>[2x]MAAKPKLYYFNGRGRMESIRWLLAAAGVEFEEEFLETREQYEKMQKDGHLLFG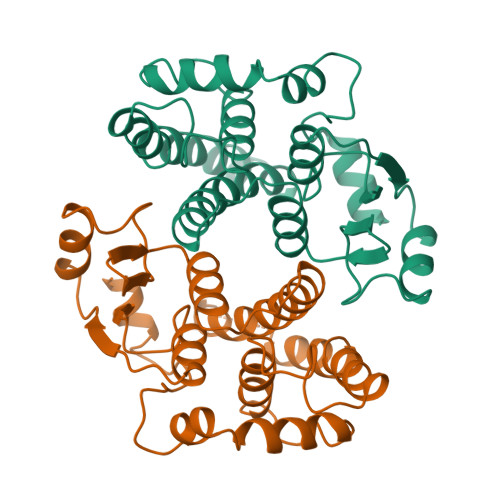QVPLVEIDGMMLTQTRAILSYLAAKYNLYGKDLKERVRIDMYADGTQDLMMMIAVAPFKTPKEKEESYDLILSRAKTRYFPVFEKILKDHGEAFLVGNQLSWADIQLLEAILMVEELSAPVLSDFPLLQAFKTRISNIPTIKKFLQPGSQRKPPPDGPYVEVVRIVLKF> MAHHHHHHMIDPNSLLPKLPSPDELKPFPTVQQTIFRGHEGRVRSVAIDPTGVALATGGDDGTVRVWELLTGRQVWSVKLNGDEAVNTVRWRPTKDTFILAAAAGEDIFLMIPTHPSVTPALDQASRDILNAGFGHATNGKQQANLPPGKEPPGKWARPGTR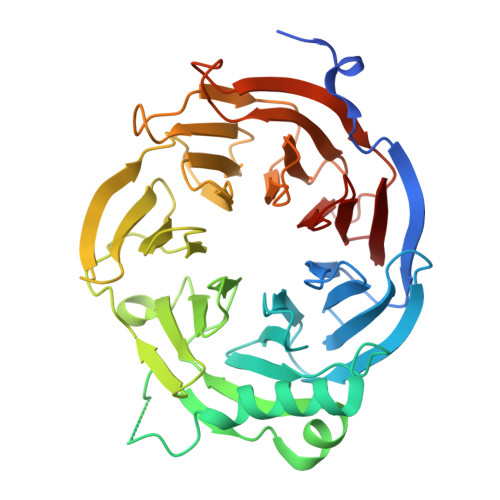LEDEGVLLRITVRSTIKAISWHRRGDHFATVSPSGQRSSVAIHTLSKHLTQIPFRKLNGLAQTASFHPLRPLFFVATQRSIRCYDLQKLELVKIVQPGAKWISSFDVHPGGDNLVVGSYDKRLLWHDLDLSNRPYKTMRFHTEAIRAVRFHKGGLPLFADASDDGSLQIFHGKVPNDQLENPTIVPVKMLKGHKVVNKLGVLDIDWHPREPWCVSAGADGTARLWM>HEDEIKKLRTSGSMTQNPHEVARVRNLNRIIMGKYEIEPWYFSPYPIELTDEDFIYIDDFTLQYFGSKKQYERYRKKCTLRHPPGNEIYRDDYVSFFEIDGRKQRTWCRNLCLLSKLFLDHKTLYYDVDPFLFYCMTRRDELGHHLVGYFSKEKESADGYNVACILTLPQYQRMGYGKLLIEFSYELSKKENKVGSPQKPLSDLGLLSYRAYWSDTLITLLVEHQKEITIDEISSMTSMTTTDILHTAKTLNILRYYKGQHIIFLNEDILDRYNRLKAKKRRTIDPNRLIWKPPVFTASQLRFAW[3x];>MTDELKSYEALKAELKKSLQDRREQEDTFDNLQQEIYDKETEYFSHNSNNNHSGHGGAHGSKSHYSGNIIKGFDTFSKSHHSHADSAFNNNDRIFSLSSATYVKQQHGQSQND[3x];>IPTPDASMTWNEYDKFYTGSFQETTSYIKFSATVEDCCGTNYNMDERDETFLNEQVNKGSSDILTEDEFEILCSSFEHAIHERQPFLSMDPESILSFEELKPTLIKSDMADFNLRNQLNHEINSHKTHFITQFDPVSQMNTRPLIQLIEKFGSKIYDYWRERKIEVNGYEIFPQLKFERPGEKEEIDPYVCFRRREVRHPRKTRRIDILNSQRLRALHQELKNAKDLALLVAKRENVSLNWINDELKIFDQRVKIKNLKRSLNISGEDDDLINHKRKRPT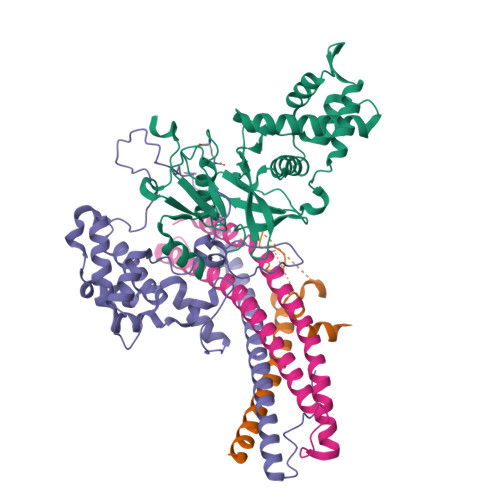[3x];>[3x]MDPSLVLEQTIQDVSNLPSEFRYLLEEIGSNDLKLIEEKKKYEQKESQIHKFIRQQGSIPKHPQEDGLDKEIKESLLKCQSLQREKCVLANTALFLIARHLNKLEKNIALLEEDGVLAPV> MELKASISDYTEAEFLQLVTTICN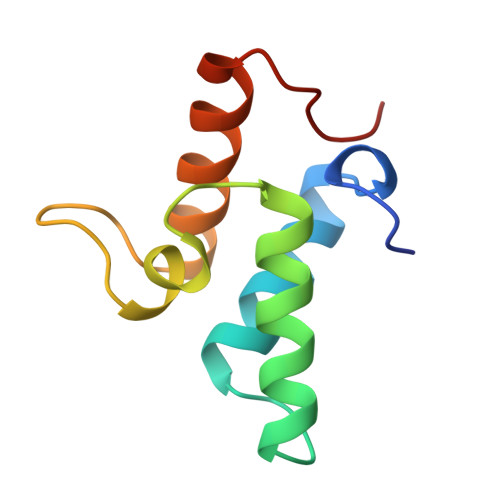ADTSSEEELVKLVTHFEEMTEHPSGSDLIYYPKEGDDDSPSGIVNTVQQWRAANGKSGFKQG>[2x]G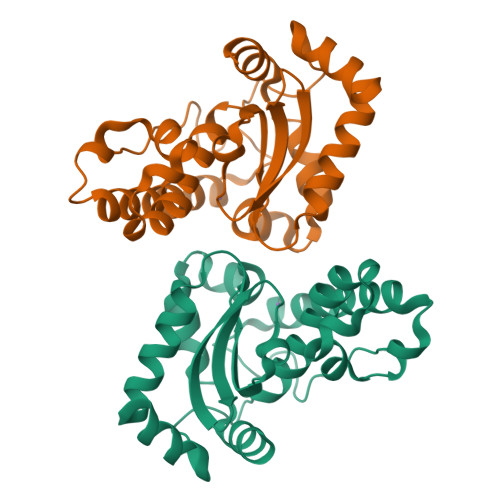SSHHHHHHMAKHELPNLPYAYDALEPHFDKETMNIHHTKHHNTYITNLNAALEGHAELADKSVEELVANLNEVPEAIRTAVRNNGGGHANHTFFWTILSPNGGGQPVGELATAIEAKFGSFDAFKEEFAKAGATRFGSGWAWLVVNNGELEVTSTPNQDSPLTEGKTPVIGLDVWEHAYYLNYQNRRPDYIGAFWNVVDWNAAEKRYQEAK> PVQLNLLYVQARDDILNGSHPVSFDKACEFAGYQCQIQFGPHNEQKHKPGFLELKDFLPKEYIKQKGERKIFMAHKNCGNMSEIEAKVRYVKLARSLKTYGVSFFLVKEKMKGKNKL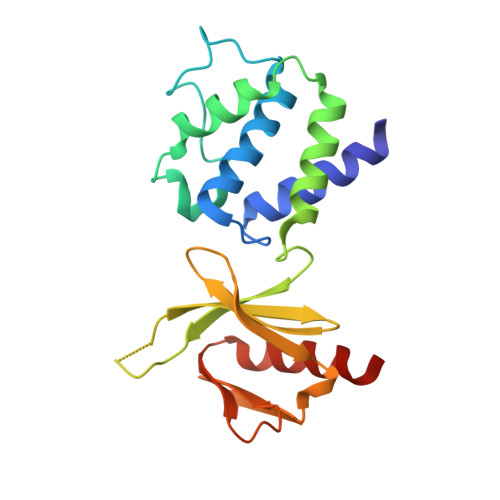VPRLLGITKECVMRVDEKTKEVIQEWSLTNIKRWAASPKSFTLDFGDYQDGYYSVQTTEGEQIAQLIAGYIDIIL>MSEEVSKNLSETLFVKHKQAKETSALTQYMPTSQSLLDEIKEKNGFSWYRNLRRLQWVWQGVDPIEQEQVLARIASSKHSRTDEQWLDTVMGYHSGNWAYEWTRLGMEHQKRAGEMTNEAASEALFSASLCYSIAGYPHLKSDNLAIQAQVLANSAYLEAAKKSKYIIKQLEIPFEKGKITAHLHLTNTDKPHPVVIVSAGLDSLQTDMWRLFRDHLAKHDIAMLTVDMPSVGYSSKYPLTEDYSRLHQAVLNELFSIPYVDHHRVGLIGFRFGGNAMVRLSFLEQEKIKACVILGAPIHDIFASPQKLQQMPKMYLDVLASRLGKSVVDIYSLSGQMAAWSLKVQGFLSSRKTKVPILAMSLEGDPVSPYSDNQMVAFFSTYGKAKKISSKTITQGYEQSLDLAIKWLEDELLR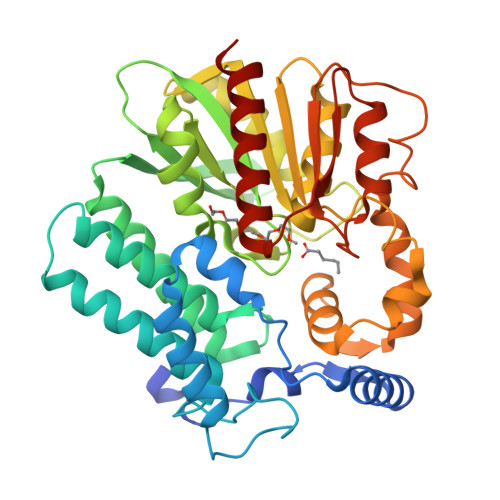[2x]> GSHMFSLITWNIDGLDLNNLSERARGVCSYLALYSP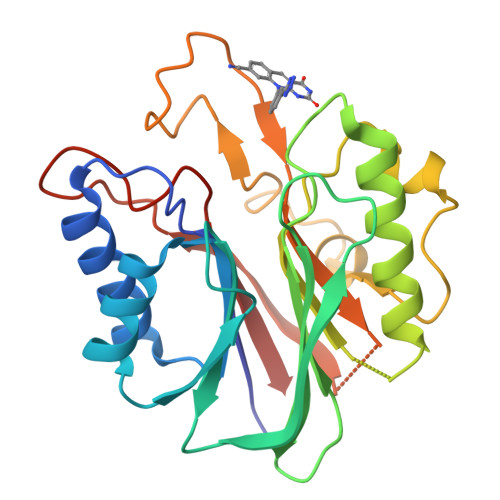DVIFLQEVIPPYYSYLKKRSSNYEIITGHEEGYFTAIMLKKSRVKLKSQEIIPFPSTKMMRNLLCVHVNVSGNELCLMTSHLESTRGHAAERMNQLKMVLKKMQEAPESATVIFAGDTNLRDREVTRSGGLPNNIVDVWEFLGKPKHCQYTWDTQMNSNLGITAACKLRFDRIFFRAAAEEGHIIPRSLDLLGLEKLDCGRFPSDHWGLLCNLDIIL>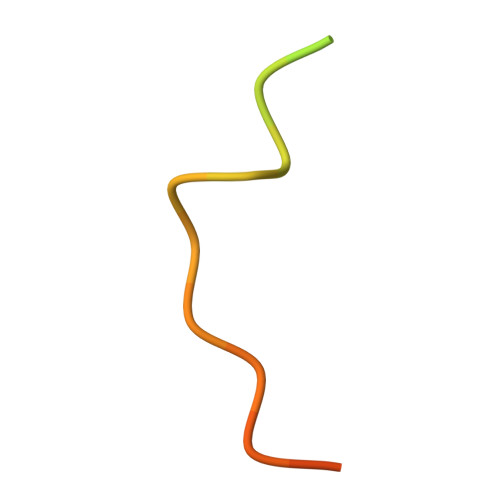 MEVQNQHAKEESLADDLFRYNPYLKRRR> MAGAPHPHTYMGWWGSLGSPKQKYITQYTISPYAAKPLKGAAYNAVFNTFRRTKNQFLYVAIPFV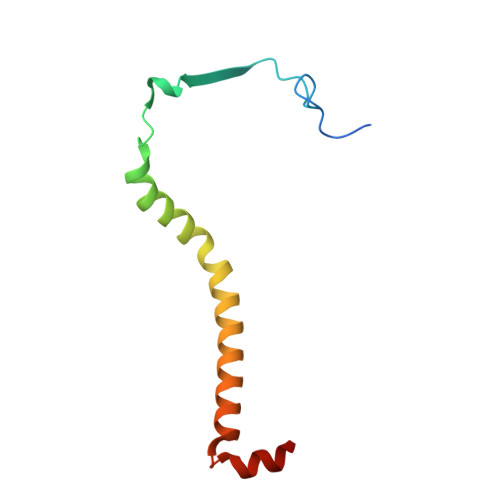VVWSIWTRARDYNEYLYTKEGREELERVNV[6-methyl-5-oxidanyl-4-[(2-phenylhydrazinyl)methyl]pyridin-3-yl]methyl dihydrogen 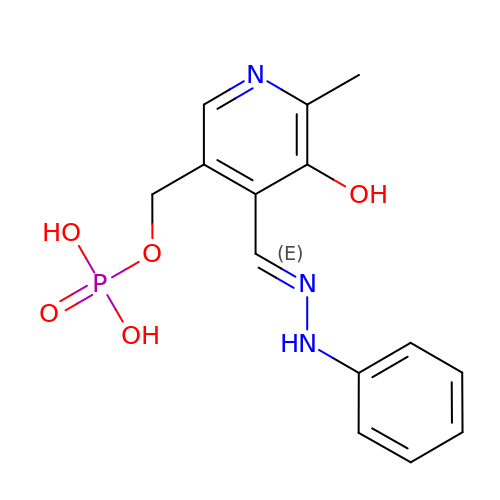phosphate | C14 H16 N3 O5 P | VZZGBIJWEDOPQL-LZYBPNLTSA-N>MKKITLLLAGSALLLSGCAGVKSSFDCDATTSDTCMTMTKANQLARDKAAKQAGKPAAGGLPSLVNLPATSAVEVPSASRSAVTPPSGTRTVSTTPPVSAGTSAGVNTNTTTSTLTPRPVAGTPVTTTPSSVAYRPVVSVVTPTPSCQNVRCDNPGTVHPQRSRDQIATVWIAPWVDSDNAFHQPGRVSFVVSPADWVLPARVN[26x];>MKNNLPAFLFGTAMMVVMPPAAQAQSPATISLPQGGQFRLSISNTDPNMIFIPGDKVTAITAPGGMLADKRLTRAGGVLFTSVATRTFTIFVETARGQTFSVVATPVKGEGRVYRLMSAEPPSRPETRKWETAQAYEKLLISLNRAVLTGDIPDGYGEVKPLSDGIRLPGGFSVTPLKAWAGDQLRADRYELRNANTWGVALREQDFWKPGVRAVMFDNNAQTLMGGGRMTVTVIRGNGEGEDGQR[26x];>MANVNKVVRRRQVALLIALVLGIGAGGAGTWMVSEMNLKKAPPAKAPKGEPAPDMTGVVNQSFDNKVQRSAIAEAQRLNKETQTEIKKLRTEMGLVSRDLKGSQDRIRELEDQNQLLQTQLEAGKNFDSLSAEPLPGALASQGKPAPAGNVPPPTSFWPAGGGQAPAAPVMTPIQRPGMMDSQEFSLPDTGPKKPRFPWISSGSFVEAIVVEGADANASVTGDKNTAPMQLRLTGKVQMPNDEEFDLTGCFVTLEAWGDVSSERAIVRSRSISCKLGDDDIDQKIAGHVSFMGKNGIKGEVVMRNGQILLYAGGAGFLDGIGKGIEKASSTTVGVGATASMSAADIGQAGLGGGVSSAAKTLSDYYIKRAEQY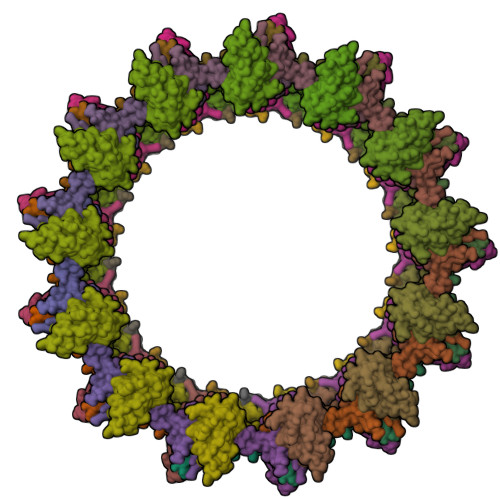HPVIPIGAGNEVTLVFQDGFQLETLEEARAKAAARKKQNQPSASSTPAAMPGNTPDMLKQLQDFRVGDTVDPATGQVVTQ[26x]>[2x]SGTVKYTDAQIQRLREYGNGTYEQKVFEDLASRDAAFSKEMSVA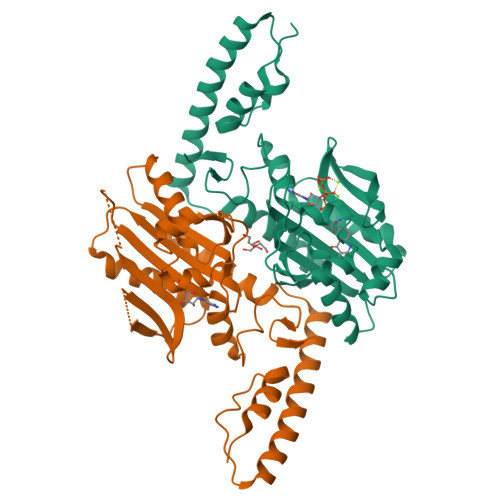STDNEKKIKGMIANPSRHGLTQLMNDIADALVAEGFIEVRTPIFISKDALARMTITEDKPLFKQVFWIDEKRALRPMLAPNLYSVMRDLRDHTDGPVKIFEMGSCFRKESHSGMHLEEFTMLSLCDMGPRGDATEVLKNYISVVMKAAGLPDYDLVQEESDVYKETIDVEINGQEVCSAAVGPHYLDAAHDVHEPTSGAGFGLERLLTIREKYSTVKKGGASISYLNGAKIN> GSHHHHHHSSGLVPRGSFNELNAINENIRDDLSALLKSDFFKYFRLDLYKQCSFWDANDGLCLNRACSVDVVEDWDTLPEYWQPEILGSFNNDTMKEADDSDDECKFLDQLCQTSKKPVDIEDTINYCDVNDFNGKNAVLIDLTANPERFTGYGGKQAGQIWSTIYQDNCFTIGETGESLAKDAFYRLVSGFHASIGTHLSKEYLNTKTGKWEPNLDLFMARIGNFPDRVTNMYFNYAVVAKALWKIQPYLPEFSFCDLVNKEIKNKMDNVISQLDTKIFNEDLVFANDLSLTLKDEFRSRFKNVTK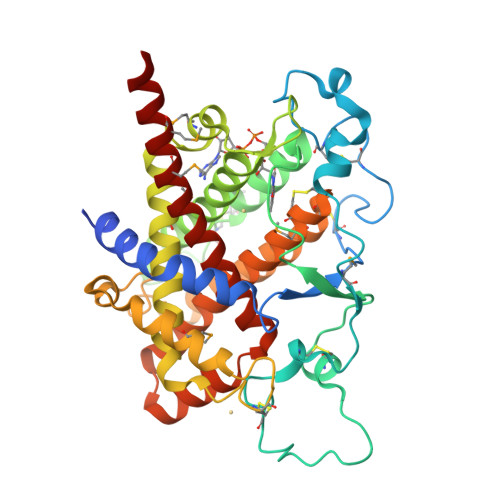IMDCVQCDRCRLWGKIQTTGYATALKILFEINDADEFTKQHIVGKLTKYELIALLQTFGRLSESIESVNMFEKMYGKRLLER> MSDMNNPSDENTGALDDLWADALNEQKATTT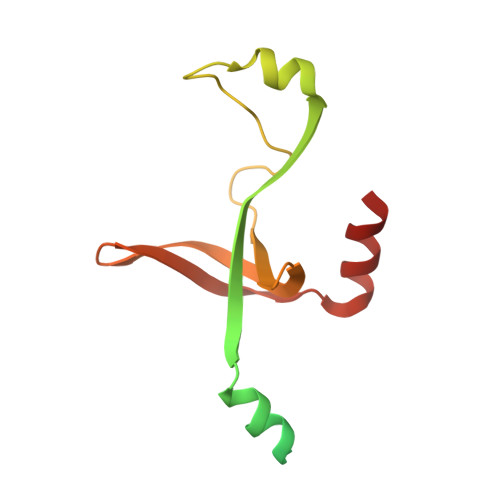KSAADAVFQQLGGGDVSGAMQDIDLIMDIPVKLTVELGRTRMTIKELLRLTQGSVVALDGLAGEPLDILINGYLIAQGEVVVVADKYGVRITDIITPSERMRRLSR>MKWMFKEDHSLEHRCVESAKIRAKYPDRVPVIVEKVSGSQIVDIDKRKYLVPSDITVAQFMWIIRKRIQLPSEKAIFLFVDKTVPQSSLTMGQLYEKEK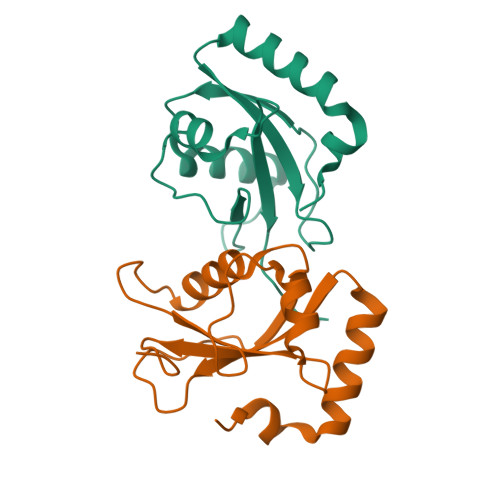DEDGFLYVAYSGENTFGF[2x]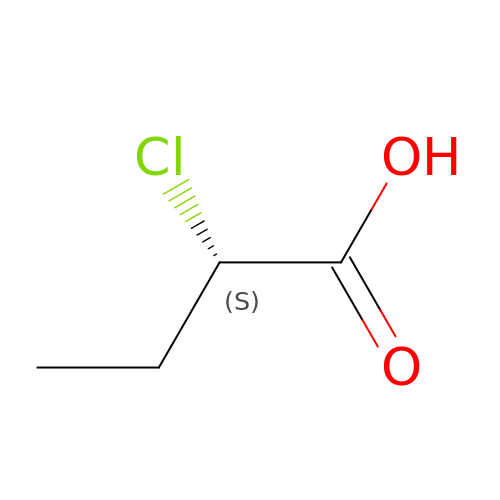(2S)-2-chlorobutanoic acid | C4 H7 Cl O2 | RVBUZBPJAGZHSQ-VKHMYHEASA-N> AAQTNAPWGLARISSTSPGTSTYYYDESAGQGSCVYVIDTGIEASHPEFEGRAQMVKTYYYSSRDGNGHGTHCAGTVGSRTYGVAKKTQLFGVKVLDDNGSGQYSTIIAGMDFVASDKNNRNCPKGVVASLSLGGGYSSSVNSAAARLQSSGVMVAVAAGNNNADARNYSPASEPSVCTVGASDRYDRRSSFSNYGSVLDIFGPGTS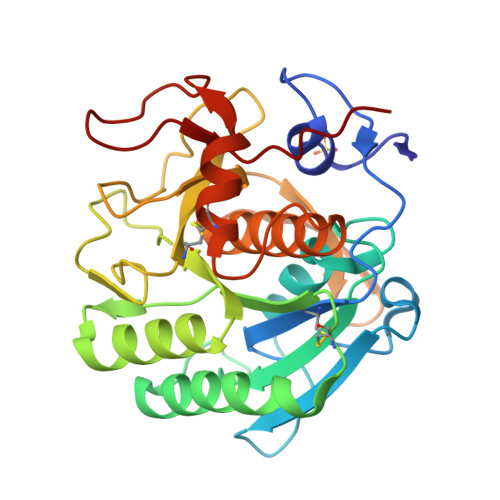ILSTWIGGSTRSISGTSMATPHVAGLAAYLMTLGKTTAASACRYIADTANKGDLSNIPFGTVNLLAYNNYQA> GLVPRGSHMTEVLHIEGHDIKVTNPDKVLFPEDGITKGELVDYYRRISGVMVPLVRGRPMTMQRFPDGIGKEGFFQKEASDYFPDWVHRATLELGKGGIQHQVVCDDAATLVYLASQAMITPHVFLSRIDKV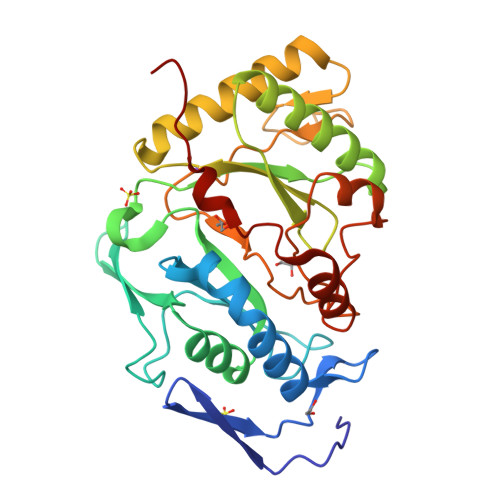HYPDRLIFDLDPPDNNFETVRSAAKTIREALDAEGYPVYLMTTGSRGLHVVVPLDRSADFDTVRAFARGFGEKLTKKYPDRFTIELSKEKRRGRLFLDYLRNSYGQTGVAPYGVRARSGAPVATPITWDELDDISGSQEYNIRNIMGRMDKRGDAWKYIDKDRTSIKNL> NQPYRTGFHFQPPKNWMNDPNGPMIYKGIYHLFYQWNPKGAVWGNIVWAHSTSTDLINWDPHPPAIFPSAPFDINGCWSGSATILPNGKPVILYTGIDPKNQQVQNIAEPKNLSDPYLREWKKSPLNPLMAPDAVNGINASSFRDPTTAWLGQDKKWRVIIGSKIHRRGLAITYTSKDFLKWEKSPEPLHYDDGSGMWECPDFFPVTRFGSNGVETSSFGEPNEILKHVLKISLADTKHDYYTIGTYDRVKDKFVPDNGFKMDGTAPRYDYGKYYASKTFFDSAKNRRILWGWTNESSSVEDDVEKGWSGIQTIPRKIWLDRSGKQ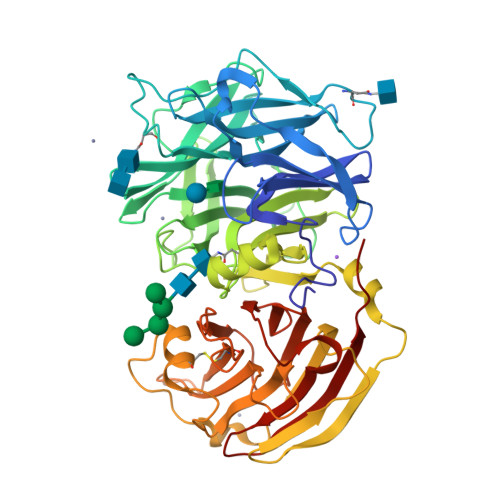LIQWPVREVERLRTKQVKNLRNKVLKSGSRLEVYGVTAAQADVEVLFKVRDLEKADVIEPSWTDPQLICSKMNVSVKSGLGPFGLMVLASKNLEEYTSVYFRIFKARQNSNKYVVLMCSDQSRSSLKEDNDKTTYGAFVDINPHQPLSLRALIDHSVVESFGGKGRACITSRVYPKLAIGKSSHLFAFNYGYQSVDVLNLNAWSMNSAQ>GAMDSSEMSTICDKTLNPSFCLKFLNTKFASPNLQALAKTTLDSTQARATQTLKKLQSIIDGGVDPRSKLAYRSCVDEYESAIGNLEEAFEHLASGDGMGMNMKVSAALDG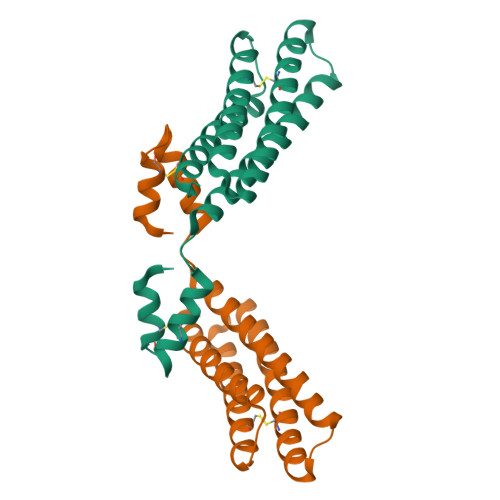ADTCLDDVKRLRSVDSSVVNNSKTIKNLCGIALVISNMLPRN[3x]> GSFTMAQQSGGGLTRGSFPEGFVFGTASAAYQYEGAVKEDGRGQTIWDTFAHTFGKITDFSNADVAVDQYHRFEEDIQLMADMGMDAYRFSIAWSRIYPNGV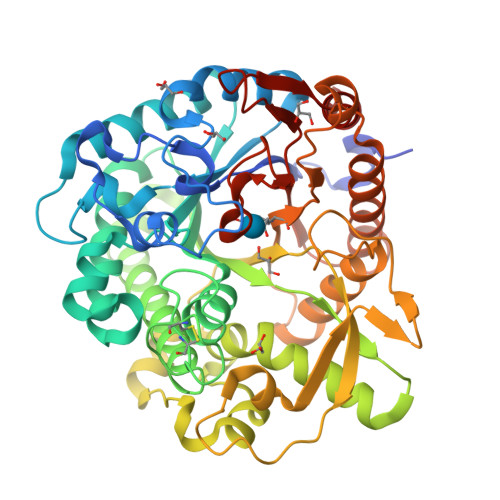GQVNQAGIDHYNKLIDALLAKGIQPYVTLYHWDLPQALEDKYKGWLDRQIVDDFAAYAETCFREFGDRVKHWITLNQPHTVAIQGYDAGLQAPGRCSVLLHLYCKAGNSGTEPYVVAHHFILAHAAAASIYRTKYKATQNGQLGIAFDVMWFEPMSNTTIDIEAAKRAQEFQLGWFADPFFFGDYPATMRARVGERLPRFTADEAAVVKGALDFVGINHYTTYYTRHNNTNIIGTLLNNTLADTGTVSLPFKNGKPIGDRANSIWLYIVPRGMRSLMNYVKERYNSPPVYITENGMDDSNNPFISIKDALKDSKRIKYHNDYLTNLAASIKEDGCDVRGYFAWSLLDNWEWAAGYSSRFGLYFVDYKDNLKRYPKNSVQWFKALLKT> DRHHHHHHKLSTPGPPLFNVSLDVAPELRWLPVLRHYDVELVRAAVAQVIGDRVPKWVLALIEKGALKLERLLPPPFTAEIRGMCDFLNLSLADGLL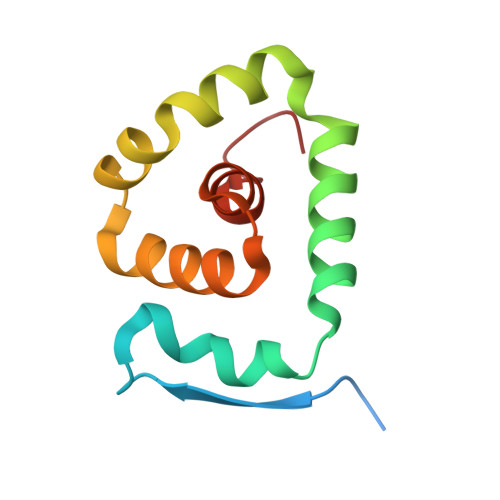VNLAYEYSAF>[5x]MAKPIITLNGLKIVIMLGMLVIILCGIRFAAEIIVPFILALFIAVILNPLVQHMVRWRVPRVLAVSILMTIIVMAMVLLLAYLGSALNELTRTLPQYRNSIMTPLQALEPLLQRVGIDVSVDQLAHYIDPNAAMTLLTNLLTQLSNAMSSIFL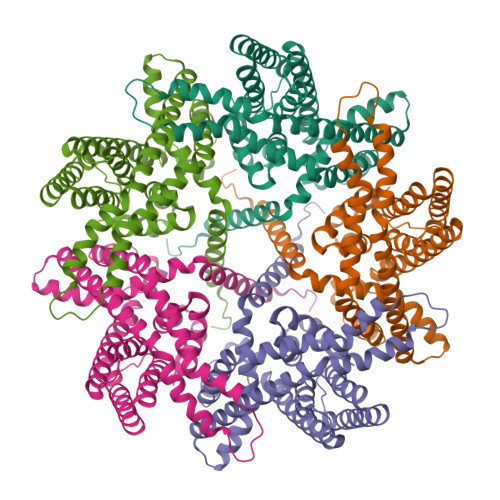LLLTVLFMLLEVPQLPGKFQQMMARPVEGMAAIQRAIDSVSHYLVLKTAISIITGLVAWAMLAALDVRFAFVWGLLAFALNYIPNIGSVLAAIPPIAQVLVFNGFYEALLVLAGYLLINLVFGNILEPRIMGRGLGLSTLVVFLSLIFWGWLLGPVGMLLSVPLTIIVKIALEQTAGGQSIAVLLSDLNKE>[2x]HMAVSGPDDYLQHSIVPTMHYQDSLPRLPIPKLEDTMKRYLNAQKPLLDDSQFRRTEALCKNFETGVGKELHAHLLAQDKQNK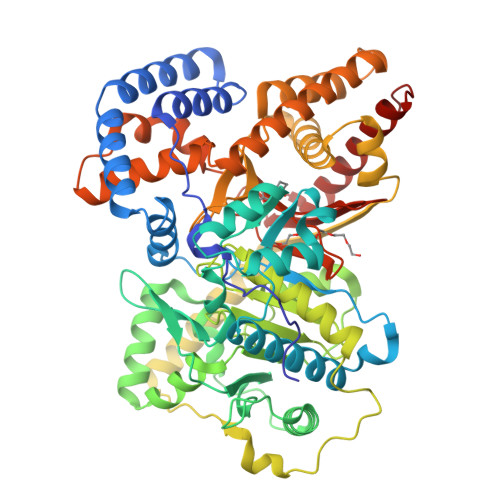HTSYISGPWFDMYLTARDSIVLNFNPFMAFNPDPKSEYNDQLTRATNLTVSAVRFLKTLQAGLLEPEVFHLNPSKSDTDAFKRLIRFVPPSLSWYGAYLVNAYPLDMSQYFRLFNSTRIPRPNRDELFTDTKARHLLVLRKGHFYVFDVLDQDGNIVNPLEIQAHLKYILSDSSPVPEFPVAYLTSENRDVWAELRQKLIFDGNEETLKKVDSAVFCLCLDDFPMKDLIHLSHTMLHGDGTNRWFDKSFNLIVAEDGTAAVHFEHSWGDGVAVLRFFNEVFRDSTQTPAITPQSQPAATNSSASVETLSFNLSGALKAGITAAKEKFDTTVKTLSIDSIQFQRGGKEFLKKKQLSPDAVAQLAFQMAFLRQYGQTVATYESCSTAAFKHGRTETIRPASIFTKRCSEAFVRDPSKHSVGELQHMMAECSKYHGQLTKEAAMGQGFDRHLYALRYLATARGLNLPELYLDPAYQQMNHNILSTSTLNSPAVSLGGFAPVVPDGFGIAYAVHDDWIGCNVSSYSGRNAREFLHCVQKCLEDIFDALEGKAIKT>MSLNPRLFSPHIIRSLLDLDAYKINMMQAIHHFYPDVSVRYELIVRSEEDASGLLDAIRQEIAHLGTLRFSDADIHYLTQHAPHLKATFLQSLRYFHFVPQEQVEMGIVKQGGKQQLRISIRGSWRDTILYETLVMAIVSEVRSRQRWAEVPADLPLKVLKTKLDQLKAEIERRGINNFSLTEMGTRRRFSSQVQRDVLACLKQEIPQWVLGTSNYHFAREFDLKPIGTIAHEWFMGHQALVNERDSQQVALERWLTAFDGMLAIAPTDTLTIDAFLNDFNRHLANAYDGVRHDSGCPFRWGDKMIAHYQQLGIDPTTKLFIFSDGLDFDQALELCEYFAGRVKISFG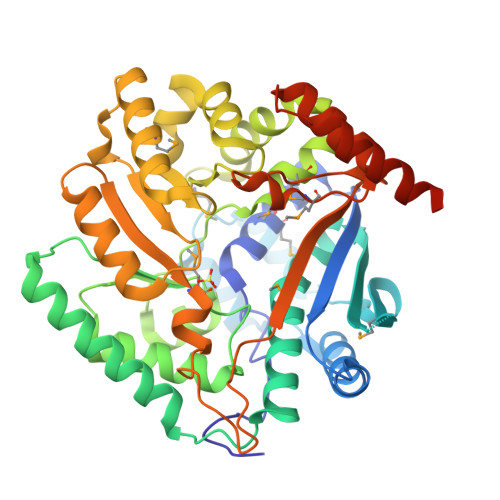IGTFLTNDLANWRNAAGVEYRPLSIVIKLAECQGRPVAKISDQPEKAMCEDPIFLANLKRRFNIELDVDALIQELRHQKRSPRHYISAAAEGHHHHHH[2x]>MWSHPAVRKSSSKTIRSRSIWDDAHAMLEKAKAEGISTVWDRAAEQTPACKFCELGTTCRNCIMGPCRIANRKDGKMRLGVCGADADVIVARNFGRFIAGGAAGHSDHGRDLIETLEAVAEGKAPGYTIRD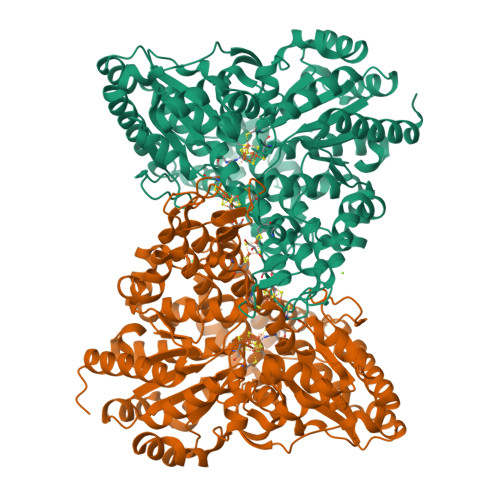VAKLRRIAAELGVADAATRPAHDVAADLVTICYNDFGSRRNALAFLARAPQVRRDLWQRLGMTPRGVDREIAEMMHRTHMGCDNDHTSLLVHAARTALADGWGGSMIGTELSDILFGTPRPRQSTVNLGVLRKDAVNILVHGHNPVVSEMILAATREPAVRQAAQDAGAADINVAGLCCTGNELLMRQGIPMAGNHLMTELAIVTGAADAIVADYQCIMPSLVQIAACYHTRFVTTSPKGRFTGATHVEVHPHNAQERCREIVMLAIDAYTRRDPARVDIPSQPVSIMSGFSNEAILEALGGTPKPLIDAVVAGQIRGFVGIVGCNNPKIRQDSANVTLTRELIRRDIMVLATGCVTTAAGKAGLLVPEAASKAGEGLAAVCRSLGVPPVLHMGSCVDNSRILQLCALLATTLGVDISDLPVGASSPEWYSEKAAAIAMYAVASGIPTHLGLPPNILGSENVTAMALHGLQDVVGAAFMVEPDPVKAADMLEAHIVARRARLGLTS[4x]> 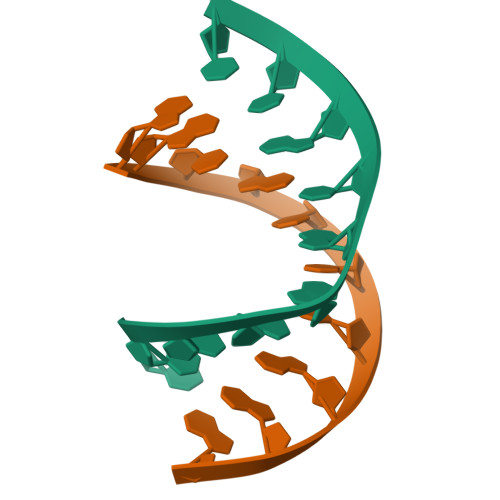UUCGGGCGCC;> GGCGCCCGAA>[8x]MNKHVNKVALIGAGFVGSSYAFALINQGITDELVVIDVNKEKAMGDVMDLNHGKAFAPQPVKTSYGTYEDCKDADIVCICAGANQKPGETRLELVEKNLKIFKGIVSEVMASGFDGIFLVATNPVDILT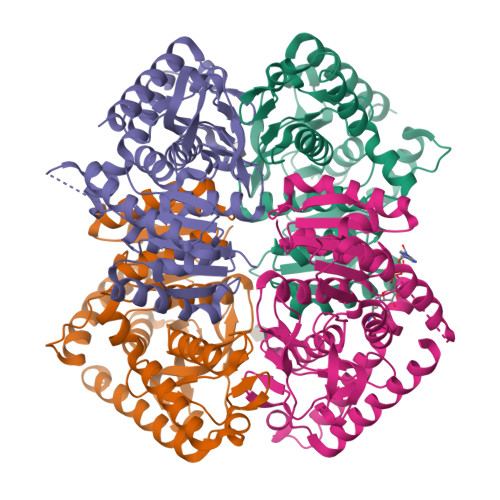YATWKFSGLPKERVIGSGTTLDSARFRFMLSEYFGAAPQNVHAHIIGEHGDTELPVWSHANVGGVPVSELVEKNDAYKQEELDQIVDDVKNAAYHIIEKKGATYYGVAMSLARITKAILHNENSILTVSTYLDGQYGADDVYIGVPAVVNRGGIAGITELNLNEKEKEQFLHSAGVLKNILKPHFAEQKVNHHHHHH> GHMNFAGKHVGFGLTGSHCTYHEVLPQMERLVELGAKVTPFVTHTVQTTDTKFGESSEWINKIKQITEEPIVDSMVKAEPFGPKTPLDCMVIAPMTGNSTSKFANAMTDSPVLMGAKATLRNGK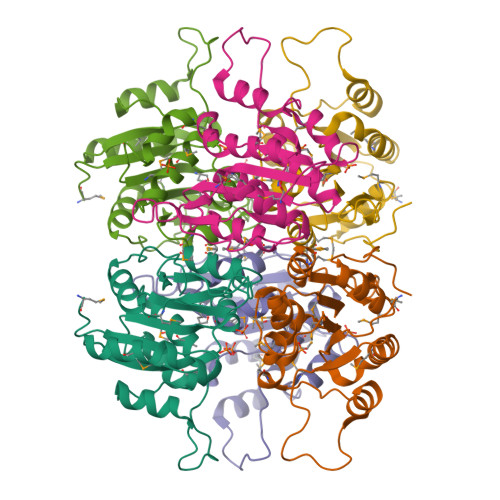PVVVGISTNDALGLNGINIMRLMATKNIYFIPFGQDNPQVKPNSLVARMEALPETIEAALRGQQYQPVLIEKFRDGS> SVTLRDLFDRAVVLSHYIHNLSSEMFSEFDKRYTHGRGFITKAINSCHTSSLATPEDKEQAQQMNQKDFLSLIVSILRSWNEPLYHLVTEVRGMQEAPEAILSKAVEIEEQTKRLLERMELIVSQVHPETKENEIYPVWSGLPSLQMADEESRLSAYYNLLHCLRRDSHKIDNYLKLLKCRIIHNNNC;> SQLPPGKPEIFKCRSPNKETFTCWWRPGTDGGLPTNYSLTYHREGETLMHECPDYITGGPNSCHFGKQYTSMWRTYIMMVNATNQMGSSFSDELYVDVTYIVQPDPPLELAVEVKQPEDRKPYLWIKWSPPTLIDLKT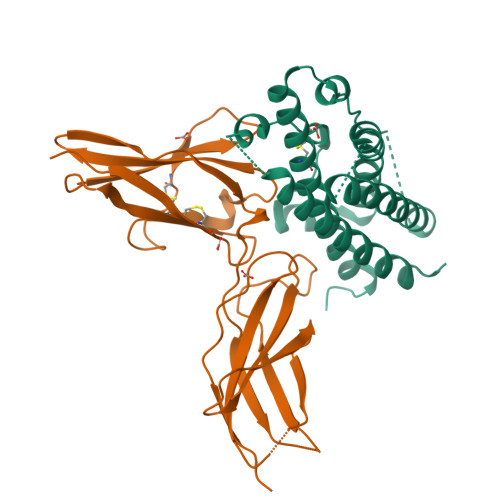GWFTLLYEIRLKPEKAAEWEIHFAGQQTEFKILSLHPGQKYLVQVRCKPDHGYWSAWSPATFIQIPSDFTMND>[8x]MDIISVALKRHSTKAFDASKKLTPEQAEQIKTLLQYSPSSTNSQPWHFIVASTEEGKARVAKSAAGNYVFNERKMLDASHVVVF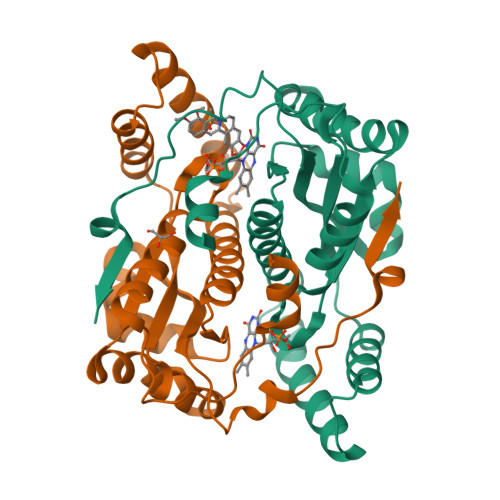CAKTAMDDVWLKLVVDQEDADGRFATPEAKAANDKGRKFFADMHRKDLHDDAEWMAKQVYLNVGNFLLGVAALGLDAVPIEGFDAAILDAEFGLKEKGYTSLVVVPVGHHSVEDFNATLPKSRLPQNITLTEV>GPGFMRDSGSKASSDSQDANQCCTSCEDNAPATSYCVECSEPLCETCVEAHQRVKYTKDHTVRSTGPAKTR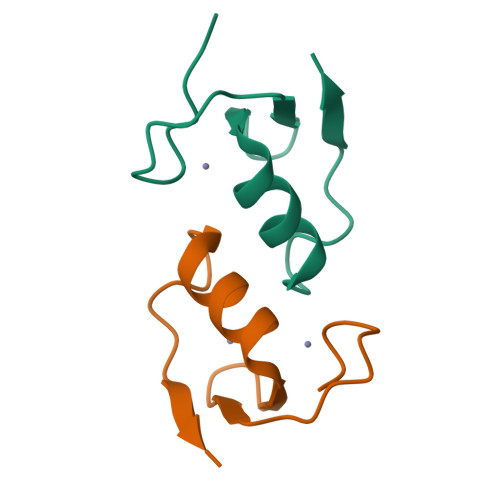D[2x]>MRGSHHHHHHTDPQGDAAQKTDTSHHDQDHPTFNKITPNLAEFAFSLYRQLAHQSNSTNIFFSPVSIATAFAMLSLGTKADTHDEILEGLNFNLTEIPEAQIHEGFQELLRTLNQPDSQLQLTTGNFLFLSEGLKLVDKFLEDVKKLYHSEAFTVNFGDTEEAKKQINDYVEKGTQGKIVDLVKELDRDTVFALVNYIFFKGKWERPFEVKDTEEEDFHVDQVTTVKVPMMKRLGMFNIQHCKKLSSWVLLMKYLGNATAIFFLPDEGKLQHLENELTHDIITKFLENEDRRSASLHLPKLSITGTYDLKSVLGQLGITKVFSNGADLSGVTEEAPLKLSKAVHKAVLTIDEKGTEAAGAMFLEAIPMSIPPEVKFNKPFVFLMIEQNTKSPLFMGKVVNPTQK[3x]

The plasma protein α1-antitrypsin is principally synthesised by hepatocytes and protects lung tissue from degradation by inhibiting neutrophil elastase. It is the archetypal member of the serpin (serine protease inhibitor) superfamily of proteins. In common with other inhibitory serpins, the native fold of α1-antitrypsin is metastable and this property is utilised in the characteristic serpin mechanism of action.

The structure of Gly117Phe α1-antitrypsin was solved to 3.2 Å resolution, allowing confident interpretation of the secondary structure of the protein. The asymmetric unit contained three molecules with minimal intermolecular contacts and in an arrangement not suggestive of biologically significant multimerisation. Electron density was not seen for residues 349–356 (copy A), 348–356 (copy B) and 348–358 (copy C) of the hypermobile reactive site loop. Before incorporation of the Phe mutation into the model or any restrained refinement had been performed, clear density was apparent at the mutation site, indicating that its side chain was oriented away from β-sheet A towards the F helix where significant changes were seen. In the refined structure, the F-helix is displaced downwards (towards the bottom of s3A) by half a turn relative to its position in the structure of native wild-type α1-antitrypsin (2.7–3.5 Å between equivalent Cα atoms). Conversely, repacking of helix F–β-sheet A interface residues, in particular Tyr160, is necessary to avoid steric clashes with the adjacent Phe117 side chain and sustain favourable hydrophobic interactions. In the refined structure of Gly117Phe α1-antitrypsin, Phe117 forms the centre of a cluster of aromatic side chains, interacting with Phe119, Phe143 and Tyr187 (all at distances of 3.5–5.5 Å). The side chain of Tyr160 is in a solvent-exposed position in this mutant in contrast to its buried position within the helix F–β-sheet A interface in wild-type α1-antitrypsin but remains well placed for aromatic interactions with two residues of this cluster, Phe119 and Phe143. The increased biochemical stability conferred by the Gly117Phe mutation on the native fold of α1-antitrypsin is therefore related to increased stabilisation of the F helix. However, stabilisation of the upper turns of the F helix and/or its downward displacement as seen in the structure of Gly117Phe α1-antitrypsin will reduce the propensity for its remodelling.>MGSLNTE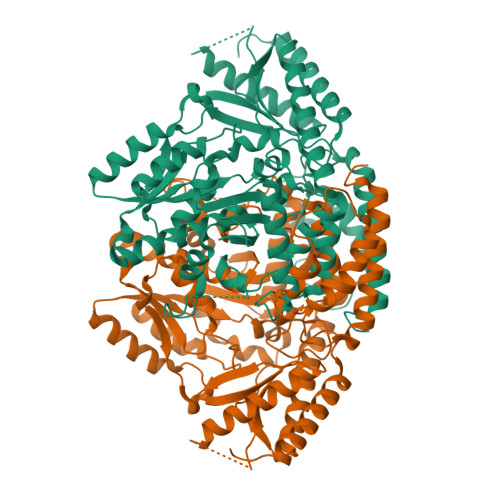DVLENSSAFGVTNPLDPEEFRRQGHMIIDFLADYYRDVEKYPVRSQVEPGYLRKRLPETAPYNPESIETILQDVTTEIIPGLTHWQSPNYYAYFPSSGSVAGFLGEMLSTGFNVVGFNWMSSPAATELESVVMDWFGKMLNLPESFLFSGSGGGVLQGTSCEAILCTLTAARDRKLNKIGREHIGRLVVYGSDQTHCALQKAAQVAGINPKNFRAIKTFKENSFGLSAATLREVILEDIEAGLIPLFVCPTVGTTSSTAVDPISPICEVAKEYEMWVHVDAAYAGSACICPEFRHFIDGVEEADSFSLNAHKWFFTTLDCCCLWVKDPSALVKALSTNPEYLRNKATESRQVVDYKDWQIALSRRFRSLKLWMVLRSYGVTNLRNFLRSHVKMAKTFEGLICMDGRFEITVPRTFAMVCFRLLPPKTIKVYDNGVHQNGNGVVPLRDENENLVLANKLNQVYLETVNATGSVYMTHAVVGGVYMIRFAVGSTLTEERHVIYAWKILQEHADLILGKFSEADFSS[6x]> MDGSGEQPRGGGPTSSEQIMKTGALLLQGFIQDRAGRMGGEAPELALDPVPQDASTKKLSESLKRIGDELDSNMELQRMIAAVDTDSPREVFFRVAADMFSDGNFNWGRVVALFYFASKL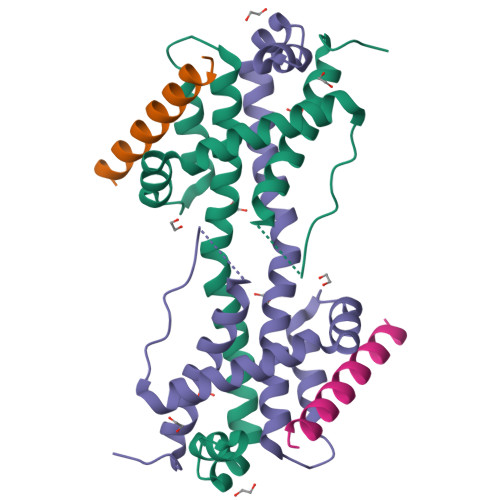VLKALSTKVPELIRTIMGWTLDFLRERLLGWIQDQGGWDGLLSYFGTPTW;> SESQEDIIRNIARHLAQVGDSMDRSIPPGLVNGL>[2x]SMETLDLLAMRE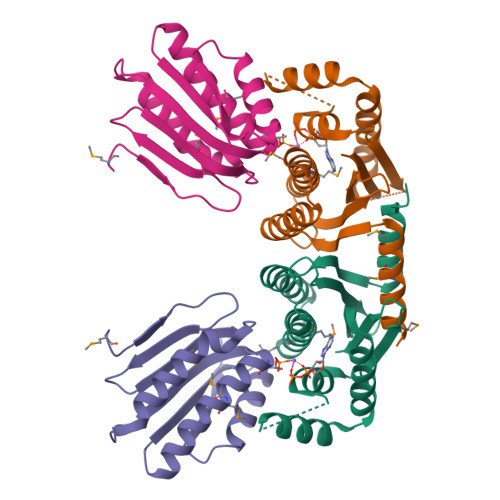SYTRQRILLCFNGPISRSLIEEIGHALRNYLHAEQAKPSEAMDVFAVYIEMTQNIRHYANLKGYGEHEAAATVAIARNEDGHYVVSAGNLVERDDGQSLVRSIQAIANLDKAALKAAYKEQLRRPRDSGCASGAGLGLLDIARKSSEPLAASLKEQPDGRAFFSLRAVI;>[2x]SMSDLHIPGTQSTPAIQGDWQAGRLSMQGDSYPENSYELFGQVIDWVERFLADGQRPLELDLRLLYLNTSSIKAMMDILDLLEEAHQGGRPVSLRWHYDRRNERVAELAEEFREDCSFPFAIQAHDE>[2x]GSHMDYLVTEEEINLTRGPSGLGFNIVGGTDQQYVSN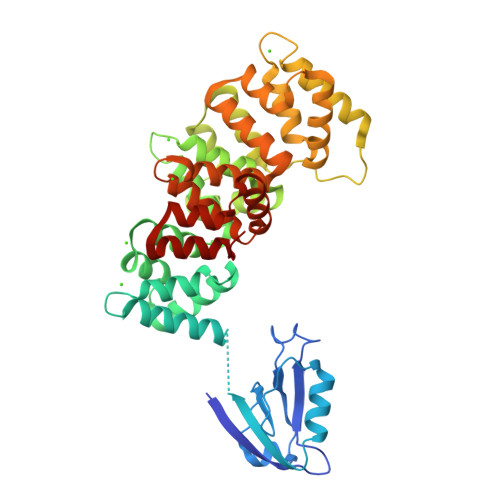DSGIYVSRIKENGAAALDGRLQEGDKILSVNGQDLKNLLHQDAVDLFRNAGYAVSLRVQHRLQVQGSAYTNFDAERDALNIETAIKTKGVDEVTIVNILTNRSNEQRQDIAFAYQRRTKKELASALKSALSGHLETVILGLLKTPAQYDASELKASMKGLGTDEDSLIEIICSRTNQELQEINRVYKEMYKTDLEKDIISDTSGDFRKLMVALAKGRRAEDGSVIDYELIDQDARDLYDAGVKRKGTDVPKWISIMTERSVPHLQKVFDRYKSYSPYDMLESIRKEVKGDLENAFLNLVQCIQNKPLYFADRLYDSMKGKGTRDKVLIRIMVSRSEVDMLKIRSEFKRKYGKSLYYYIQQDTKGDYQKALLYLCGGDD;> SEKHFRETEV Here, we develop a general method for designing self-assembling proteins that uses predicted structures of oligomeric proteins from thermophilic organisms as building blocks. Of the 359 identified thermophilic trimer homologs, 191 yielded high-confidence AF2 predictions [predicted aligned error (pAE) < 5, predicted local distance difference test (pLDDT) > 90]. We docked these predicted structures in the so-called “I3” architecture by aligning their threefold symmetry axes to the corresponding axes of icosahedral point group symmetry, using the Rosetta SymDofMover to sample the translational and rotational degrees of freedom along this shared axis [Fig. 1C, (27)]. To evaluate the accuracy of our design method at high resolution, we used single-particle cryoelectron microscopy (cryo-EM) to determine the structures of one nanoparticle from each of the successful PDB seeds.

Icosahedral 3D reconstructions at 2.5 Å, 2.3 Å, and 3.5 Å resolution were obtained for I3-A6, I3-D12, and I3-A7, respectively, allowing us to build atomic models of each nanoparticle. Comparing the experimental cryo-EM structures to the computational design models demonstrated that AF2 structure prediction was quite accurate: The all-atom rmsd for a single monomer of I3-A6, I3-D12, and I3-A7 were 1.3 Å, 1.7 Å, and 1.4 Å, respectively. Aligning two subunits across the designed interfaces revealed that these were designed with high accuracy, yielding alpha-carbon rmsds of 0.7 Å, 1.1 Å, and 1.5 Å, respectively. In each case, the rotameric states of the interdigitated hydrophobic side chains at the designed interfaces corresponded well with the design models, as did the polar residues lining the periphery of the I3-A6 and I3-D12 interfaces. Several of the polar residues at the I3-A7 interface adopted unintended rotamers, likely due to small shifts in the backbones of the loops that make up the interface. Nevertheless, essentially all of the polar and nonpolar contacts at each interface recapitulated those in the design models. Slight rigid body deviations between the building blocks added up to alpha-carbon rmsds of 1.6 Å, 2.2 Å, and 2.2 Å across the entire 60-subunit nanoparticle for I3-A6, I3-D12, and I3-A7, respectively. We found that only one of our six designed nanoparticles (I3-A7) successfully secreted from transfected Expi293F cells when an N-terminal signal peptide was appended, so our subsequent engineering efforts focused on this nanoparticle. Second we circularly permuted the subunit of I3-A7 so that its N terminus was present on the exterior of the nanoparticle and available for genetic fusion. Third, we engineered an oligomannose-type N-linked glycan into the I3-A7 subunit, as these have been shown to improve the trafficking and immunogenicity of particulate immunogens.

>[60x]MGAIVVTGIPGVGKTTVMQKAAEGSPLPRVPLEGVMYGVAKRMGLVKDIDEMRRLSPDVQKEVQKKAAERIAALGDVILDTHCTIKTPKGYLPGLPRWVLEKLRPSVILLVEADPKEIYGRRLKDETRNRDPDSEEEIAEHQMMNRAAAMAYASLSGATVKIVFNHDNRLDDAVRDAAPVLGNLEHHHHHH>[2x]SNAVGQFANFVDLLQYRAKLQARKTVFSFLADGEAESAALTYGELDQKAQAIAAFLQANQAQGQRALLLYPPGLEFIGAFLGCLYAGVVAVPAYPPRPNKSFDRLHSIIQDAQAKFALTTTELKDKIADRLEALEGTDFHCLATDQVELISGKNWQKPNISGTDLAFLQYTSGSTGDPKGVMVSHHNLIHNSGLINQGFQDTEASMGVSWLPPYHDMGLIGGILQPIYVGITQILMPPVAFLQRPFRWLKAINDYRVSTSGAPNFAYDLCASQITPEQIRELDLSCWRLAFSGAEPIRAVTLENFAKTFATAGFQKSAFYPCYGMAETTLIVSGGNGAAQLPQEIIVSKQGIEANQVRPAQGTETTVTLVGSGEVIGDQIVKIVDPQALTECTVGEIGEVWVKGESVAQGYWQKPDLTQQQFQGNVGAETGFLRTGDLGFLQGGELYITGRLKDLLIIRGRNHYPQDIELTVEVAHPAL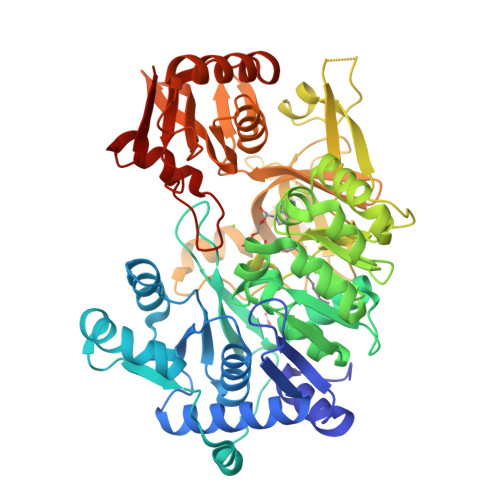RQGAGAAVSVDVNGEEQLVIVQEVERKYARKLNVAAVAQAIRGAIAAEHQLQPQAICFIKPGSIPKTSSGKIRRHACKAGFLDGSLAVVGEWQ>QGHMSNFLAEQYERDRKAIINCCFSRPDHKTGEPPNNYITHVRIIEDSKFPSSRPPPDSKLENKKKRLLILSAKPNNAKLIQIHKARENSDGSFQIGRTWQLTELVRVEKDLEISEGFILTMSKKYYWETNSAKERTVFIKSLITLYIQTFEGHVPELVNWDLSLFYLDERSYQRAVITNRPGSVSPIKSPTSNFTTNTTQSVGSVPFSAPTERTRRSETESVNPVSTPASVEYHAGMKSLNKAPYSSNS[2x];>GSHMMSNANPYENNNPYAENYEMQEDLNNAPTGHYEGSDDFVAFMNKINSINANLSRYENIINQIDAQHKDLLTQVSEEQEMELRRSLDDYISQATDLQYQLKADIKDAQRDGLHDSNKQAQAENCRQKFLKLIQDYRIIDSNYKEESKEQAKRQYTIIQPEATDEEVEAAINDVNGQQIFSQALLNANRRGEAKTALAEVQARHQELLKLEKTMAELTQLFNDMEELVIEQQENVDVIDKNVEDAQQDVEQGVGHTNKAVKSARKARKNKIRC[2x]

The final step of exocytosis in yeast involves the assembly of two t-SNAREs, Sso1/2 and Sec9, with the v-SNARE, Snc1/2, on secretory vesicles. The exocytic vesicle-docking site in yeast is marked by the octameric exocyst complex, which belongs to the CATCHR family of multi-subunit tethering proteins. Our previous work showed that one of the exocyst components, Sec3, promotes SNARE assembly by interacting with the t-SNARE Sso2. Like syntaxin-1 and other related t-SNAREs, Sso2 consists of four helices, with the first three (Habc) forming an inhibitory domain and the last (H3) serving as the SNARE motif that interacts with the other two SNAREs during membrane fusion.

Recently, we crystallized another complex of the two proteins using a longer version of Sso2 (aa1–270), which contains all Sso2 sequence except for its C-terminal transmembrane part, together with a shorter Sec3 PH domain (aa75–260). Diffraction data to 2.19 Å resolution was collected at the ESRF synchrotron site and the crystal structure was determined by the molecular replacement method. The final model contains two copies of the Sso2/Sec3 complex per asymmetric unit, together with 418 ordered water molecules. One of the complexes contains residues 4–8, 33–149, and 197–226 of Sso2 and residues 76–250 of Sec3; the other contains residues 6–14, 33–148, and 196–226 of Sso2 and residues 76–250 of Sec3. Our crystal structure of this Sec3/Sso2 complex reveals a previously unknown binding site for Sec3 on Sso2 in addition to the one on its four-helix bundle as reported in our previous work. This extra binding site is located at the N-terminal end of Sso2 and consists of two highly conserved NPY (i.e. Asn-Pro-Tyr) motifs. The NPY motifs are connected to the highly conserved helical core of Sso2 via a non-conserved linker with variable lengths (roughly 15–40 residues), which is invisible in our crystal structure, suggesting that it is mobile within the crystal structure. In the two heterodimeric complexes present in the crystal structure, the two NPY motifs of the two Sso2 molecules bind individually to a similar conserved hydrophobic pocket on the two Sec3 molecules. Particularly, the tyrosine residues in both cases (i.e. Y7 and Y13) are docked into a conserved hydrophobic pocket on the concave surface on Sec3. Overall, the NPY motif adopts a T-shaped conformation, with its broad top part shaped by the asparagine (N) and the proline (P) residues, which is stabilized by a hydrogen bond between the carboxyl group of the asparagine and the amide proton of the proline.>[4x]SNANYMETGDQRFGDLVFRQLAPNVWQHTSYLDMPGFGAVASNGLIVRDGGRVLVVDTAWTDDQTAQILNWIKQEINLPVALAVVTHAHQDKMGGMDALHAAGIATYANALSNQLAPQEGMVAAQHSLTFAANGWVEPATAPNFGPLKVFYPGPGHTSDNITVGIDGTDIAFGGCLIKDSKAKSLGNLGDADTEHYAASARAFGAAFPKASMIVMSHSAPDSRAAITHTARMADKLR

NDM-1 has been reported to be a highly potent carbapenem-hydrolyzing, zinc-dependent MBL. NDM-1 is an extended spectrum zinc dependent β-lactamase capable of hydrolyzing nearly all classes of β-lactams, impairing the ability to treat life-threatening infections with intravenously and orally available carbapenems.. NDM-1 resembles the common β-lactamase fold, although it shows low sequence similarity to β-lactamases deposited in PDB (20–33% sequence identity). Our results show that NDM-1 is unique among other MBLs due to its enlarged and flexible active site, and explain the observed extended spectrum β-lactamase activity.

The structure of mZnNDM-1 Δ36NY was obtained in the presence of 10 mM zinc chloride. The structure contains one zinc atom bound in the active site to the metal site 1 (Zn1) (see below). Indeed, zinc was found bound to the Zn1 site in the crystal structure of NDM-1 obtained in the presence of zinc chloride. All four monomers in the asymmetric unit contain zinc atoms bound to the Zn1 site (His120, His122 and His189), therefore confirming NDM-1 as a member of subclass B1 of MBLs and showing that Zn1 is a higher affinity site, as predicted for other MBLs. This zinc atom is shifted approximately 0.8 Å as compared with the di-zinc NDM-1 structure and shows somewhat longer Zn-His distances. The metal bound structure is very similar to apo structures (for example, rmsd between Cα atoms of apoNDM-1 Δ38 comparing 218 residues of chain B of mZnNDM-1 Δ36NY is 0.46 Å). In the mZnNDM-1 Δ36NY structures, there are several water molecules near the zinc atom. Monomer C contains tightly coordinated water (H-bond distance 2.8 Å) that may correspond to the position of the catalytic water molecule involved in β-lactam hydrolysis. It seems that there are three distinct states of the NDM-1: metal free, singly metalated and doubly metalated. All these states could be targeted for structure-based inhibitor design.>MDTTTATTARTDTLLQLDNQLCFALYSANLAMHKLYRGLLKALDLTYPQYLVMLVLWETDERSVSEIGERLYLDSATLTPLLKRLQAAGLVTRTRAASDERQVIIALTETGRALRSKAGAVPEQVFCASASS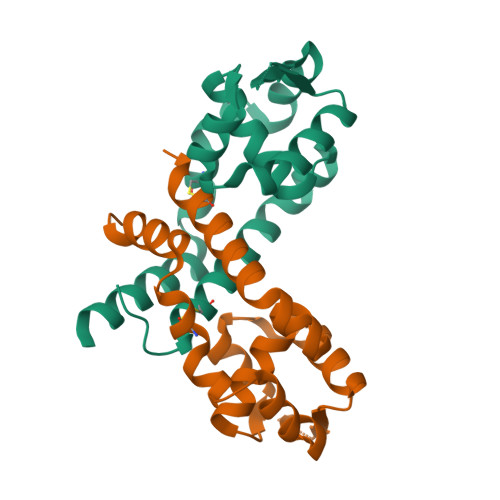LDELRQLKQELEKLRSSLGAG[2x]> GSSMASANLEGDALHTLRVTLVDPNNVLQSWDPTLVNPCTWF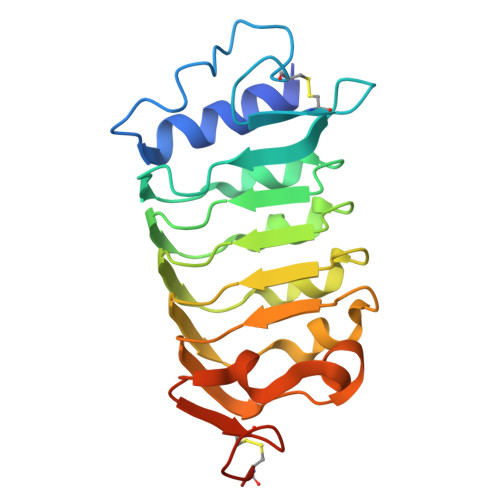HVTCNNENSVIRVDLGNAELSGHLVPELGVLKNLQYLELYSNNITGPIPSNLGNLTNLVSLDLYLNSFSGPIPESLGKLSKLRFLRLNNNSLTGSIPMSLTNITTLQVLDLSNNRLSGSVPDNGSFSLFTPISFANNLDLCGPVTSHPCPGSLENLYFQ>[2x]RADPDPMKNTCKLLVVADHRFYRYMGRGEESTTTNYLIELIDRVDDIYRNTAWDNAGFKGYGIQI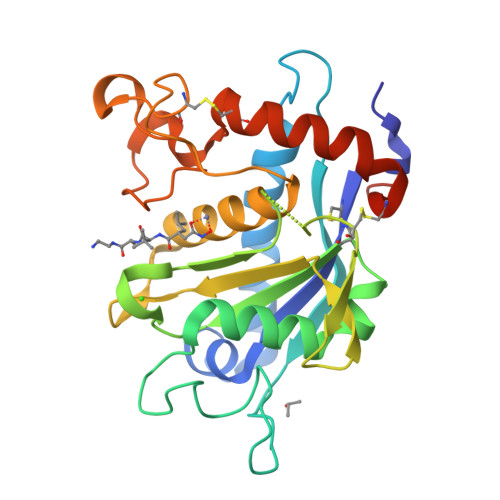EQIRILKSPQEVKPGEKHYNMAKSYPNEEKDAWDVKMLLEQFSFDIAEEASKVCLAHLFTYQDFDMGTLGLAYGGSPRANSHGGVCPKAYYSPVGKKNIYLNSGLTSTKNYGKTILTKEADLVTTHELGHNFGAEHDPDGLAECAPNEDQGGKYVMYPIAVSGDHENNKMFSQCSKQSIYKTIESKAQECFQERSNKGSHHHHHH> EQVSA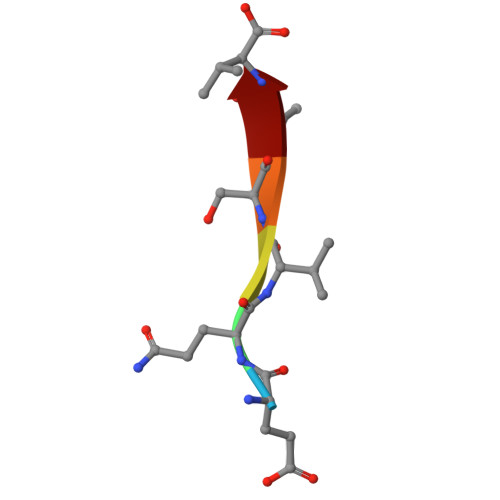V>MKRSLRKMWRPGEKKEPQGVVYEDVPDDTEDFKESLKVVFEGSAYGLQNFNKQKKLKRCDDMDTFFLHYAAAEGQIELMEKITRDSSLEVLHEMDDYGNTPLHCAVEKNQIESVKFLLSRGANPNLRNFNMMAPLHIAVQGMNNEVMKVLLEHRTIDVNLEGENGNTAVIIACTTNNSEALQILLKKGAKPCKSNKWGCFPIHQAAFSGSKECMEIILRFGEEHGYSRQLHI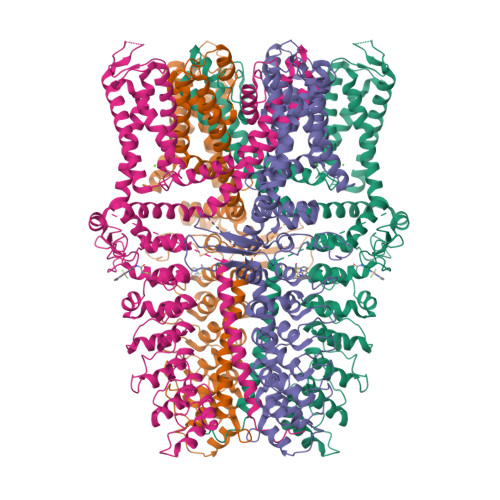NFMNNGKATPLHLAVQNGDLEMIKMCLDNGAQIDPVEKGRCTAIHFAATQGATEIVKLMISSYSGSVDIVNTTDGCHETMLHRASLFDHHELADYLISVGADINKIDSEGRSPLILATASASWNIVNLLLSKGAQVDIKDNFGRNFLHLTVQQPYGLKNLRPEFMQMQQIKELVMDEDNDGCTPLHYACRQGGPGSVNNLLGFNVSIHSKSKDKKSPLHFAASYGRINTCQRLLQDISDTRLLNEGDLHGMTPLHLAAKNGHDKVVQLLLKKGALFLSDHNGWTALHHASMGGYTQTMKVILDTNLKCTDRLDEDGNTALHFAAREGHAKAVALLLSHNADIVLNKQQASFLHLALHNKRKEVVLTIIRSKRWDECLKIFSHNSPGNKCPITEMIEYLPECMKVLLDFCMLHSTEDKSCRDYYIEYNFKYLQCPLEFTKKTPTQDVIYEPLTALNAMVQNNRIELLNHPVCKEYLLMKWLAYGFRAHMMNLGSYCLGLIPMTILVVNIKPGMAFNSTGIINETSDHSEILDTTNSYLIKTCMILVFLSSIFGYCKEAGQIFQQKRNYFMDISNVLEWIIYTTGIIFVLPLFVEIPAHLQWQCGAIAVYFYWMNFLLYLQRFENCGIFIVMLEVILKTLLRSTVVFIFLLLAFGLSFYILLNLQDPFSSPLLSIIQTFSMMLGDINYRESFLEPYLRNELAHPVLSFAQLVSFTIFVPIVLMNLLIGLAVGDIADVQKHASLKRIAMQVELHTSLEKKLPLWFLRKVDQKSTIVYPNKPRSGGMLFHIFCFLFCTGEIRQEIPNADKSLEMEILKQKYRLKDLTFLLEKQHELIKLIIQKMEIISETEDDDSHCSFQDRFKKEQMEQRNSRWNTVLRAVKAKTHHLEP[4x]>[2x]MATNGMRPIHPGEILRDEF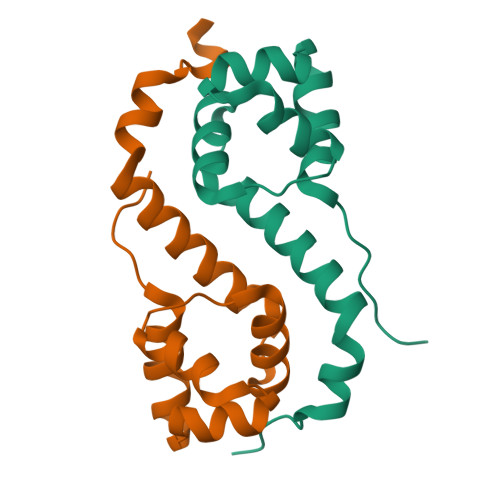LMEFDISPAALARALKVSAPTVNDIVREQRGISADMAIRLGRYFDTSAQFWMNLQSEYSLATAYAANGKQIEHEIEPLLAHG>[6x]KTVFHLGVTEADLNGATLAIIPGDPARVQKIAELMDNPVFLASHREYTVYRAELDGQSVVVCSTGIGGPSTSIAVEELAQLGVRTFLRVGTTGA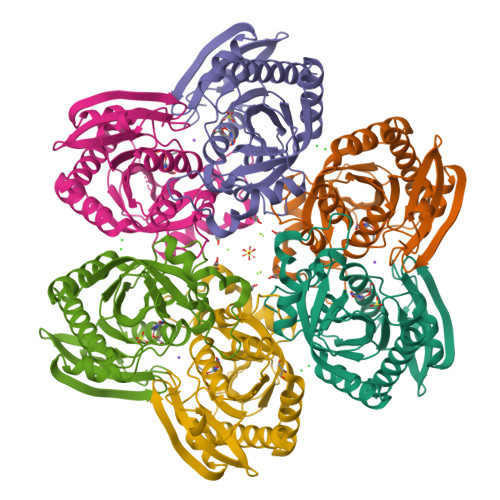IQPHVNVGDMIVTTGSVRLDGASLHFAPMEFPAVPDFDVATAMKAAAQESGATVHMGVTASSDTFYPGQERYDTFTGRVVRRFQGSMKEWQDMGVLNFEMESATLLTMCASSGLKAGCVAGVIINRTQKEIPDHATLKETEARSIKVVVEAARKMLK>[6x]MHHHHHHSSGRENLYFQGTIDDLFIFKRKLGSGAFGDVHLVEERSSGLERVIKTINKDRSQVPMEQIEAEIEVLKSLDHPNIIKIFEVFEDYHNMYIVMETCEGGELLERIVSAQARGKALSEGYVAELMKQMMNALAYFHSQHVVHKDLKPENILFQDTSPHSPIKIIDFGLAELFKSDEHSTNAAGTALYMAPEVFKRDVTFKCDIWSAGVVMYF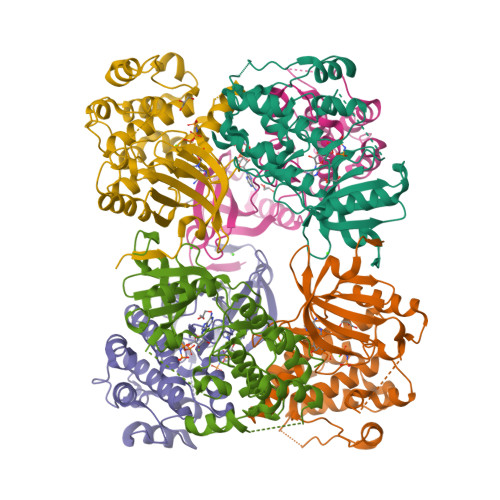LLTGCLPFTGTSLEEVQQKATYKEPNYAVECRPLTPQAVDLLKQMLTKDPERRPSAAQVLHHEWFKQA In this work, we present the production of a recombinant lectin from Tepary bean (rTBL-1) by using P. pastoris engineering, its biochemical characterization, crystallographic structure, and an analysis of its specificity for cancer-type glycans. The taxa inferred by the evolutionary analysis showed that TBL-1 belongs to the group of phytohemagglutinins of the Phaseolus genus; more specifically, the data suggest that TBL-1 is actually a homologue of PHA:L, a leucoagglutinin from Phaseolus vulgaris, present in four of the five different populations of PHA heterotetramers (E4, E3L, E2L2, EL3, and L4). The absence or the elongation of the glycosylation, if produced in other heterologous expression systems, could affect the overall folding and functionality of the protein. rTBL-1 recognizes β1-6 branched N-glycans, which are overrepresented in several types of cancer, including colon cancer.

The crystal space group was found to be P1, and the asymmetric unit contained an rTBL-1 homo-tetramer composed of two antiparallel dimers. Each monomer was composed of 15 antiparallel β-strands arranged in the classical β-sandwich or jellyroll fold observed for legume lectins such as in the case of their homologous PHA-E, PHA-L, SBA, PNA, ConA, and LOL, among others. The jellyroll fold consists of (1) a “back-sheet” with six β-strands, (2) a concave seven-stranded “front-sheet”, and (3) two “stranded-top” connecting sheets. The tetramer was obtained from the back-to-back association of both dimers stabilized through interactions between the β-strands 10 (amino acids 186–194) of the corresponding chains (Figure 4AIII). Two divalent cations, calcium Ca2+ and manganese Mn2+, are attached to each protomer through coordination with Asp131, Glu129, Asp139, His144, Leu133, and Asn135 as well as two structural water molecules per ion. They are located at the top of the “front sheet” in the vicinity of the predicted carbohydrate binding site and are indispensable for lectin activity. In accordance with the mass spectrometry data, we observed electron density that corresponds to the N-glycosylation site at Asn19. This permitted to build the proximal and the distal GlcNAc of the common core of N-glycans in all chains as well as six and four additional residues belonging to the antennas of chains A and D, respectively. No structural evidence was found to suggest that the binding pockets could be affected by the presence and/or size of this posttranslational modification.

>EAEAAASANDISFNFQRFNETNLILQGDASVSSSGQLRLTNLNDNGEPTLSSLGRAFYSTPIQIWDSTTGAVASFATSFTFNIRVPNNAGPADGLAFALVPVGSKPKDRGGLLGLFDGSDSKAHTVAVEFDTLYNRDWDPRERHIGIDVNSIKSIKTTPWDFVNGEDAEVLITYDSSTKLLVASLVYPSQKTSFIVSDTVDLKSVLPEWVSVGFSATSGISKGNVETNDLLSWSFASKLSDGTTSEGLNHHHHHH[4x]>[4x]ADKLPYKVADIGLAAWGRKALDIAENEMPGLMRMREMYSASKPLKGARIAGCLHMTVETAVLIETL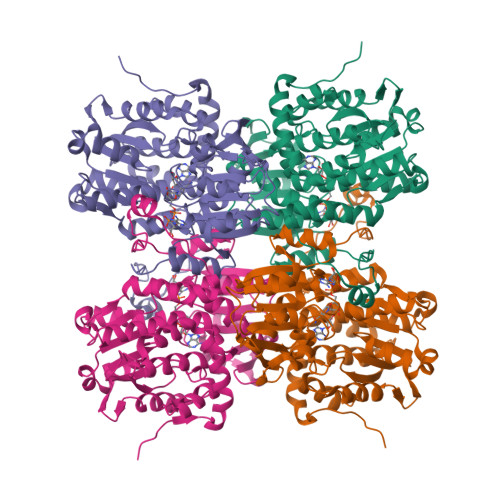VALGAEVRWSSCNIFSTQDHAAAAIAKAGIPVFAWKGETDEEYLWCIEQTLHFKDGPLNMILDDGGDLTNLIHTKHPQLLSGIRGISEETTTGVHNLYKMMANGILKVPAINVNDSVTKSKFDNLYGCRESLIDGIKRATDVMIAGKVAVVAGYGDVGKGCAQALRGFGARVIITEIEPINALQAAMEGYEVTTMDEACKEGNIFVTTTGCVDIILGRHFEQMKDDAIVCNIGHFDVEIDVKWLNENAVEKVNIKPQVDRYLLKNGHRIILLAEGRLVNLGCAMGHPSFVMSNSFTNQVMAQIELWTHPDKYPVGVHFLPKKLDEAVAEAHLGKLNVKLTKLTEKQAQYLGMPINGPFKPDHYRY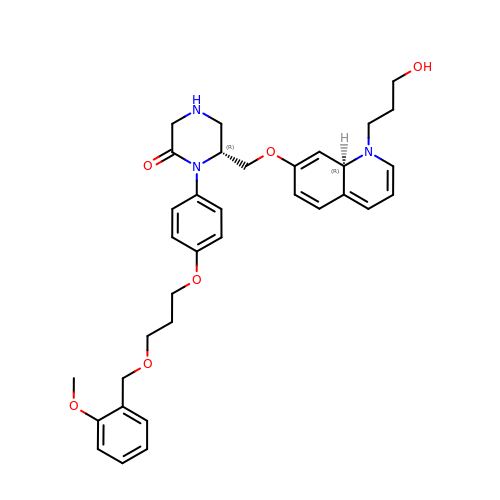(6R)-6-({[1-(3-HYDROXYPROPYL)-1,7-DIHYDROQUINOLIN-7-YL]OXY}METHYL)-1-(4-{3-[(2-METHOXYBENZYL)OXY]PROPOXY}PHENYL)PIPERAZIN-2-ONE | C34 H41 N3 O6 | BSWXEYZBVSQHOV-UYEDPJPISA-N>SYYQRSDWTADEEQILLGPFDYLESLPGKNMRSQLIQSFNTWLKVPTESLDVIIKVISMLHTASLLIDDIQDQSILRRGQPVAHSIFGTAQAMNSGNYVYFLALREVQKLQNPKAISIYVDSLIDLHRGQGMELFWRDSLMCPTEEQYLDMV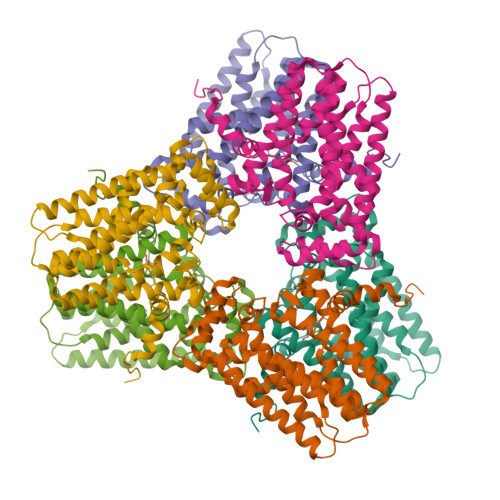ANKTGGLFCLAIQLMQAEATIQVDFIPLVRLLGIIFQICDDYLNLKSTAYTDNKGLCEDLTEGKFSFPIIHSIRSNPGNRQLINILKQKPREDDIKRYALSYMESTNSFEYTRGVVRKLKTEAIDTIQGLEKHGLEENIGIRKILARMSLEL[2x]>MTVQMEYEKDVKVAALDGKKIAVIGYGSQGHAHAQNLRDSGRDVIIGVRPGKSFDKAKEDGFDTYTVAEATKLADVIMILAPDEIQQELYEAEIAPNLEAGNAVGFAHGFNIHFEFIKVPADVDVFMCAPKGPGHLVRRTYEEGFGVPALYAVYQDATGNAKNIAMDWCKGVGAARVGLLETTYKEETEEDLFGSQAVLCGGLTALIEAGFEVLTEAGYAPELAYFEVLHEMKLIVDLIYEGGFKKMRQSISNTAEYGDYVSGPRVITEQVKEN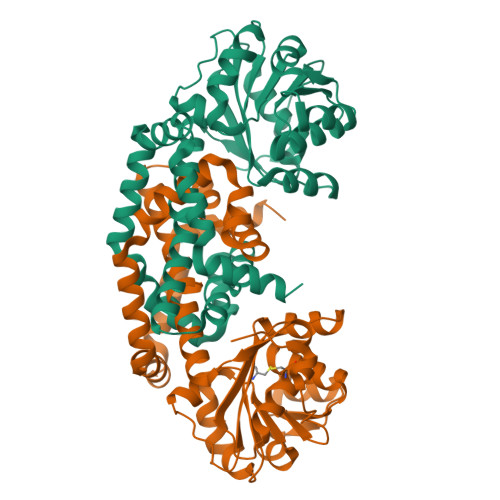MKAVLADIQNGKFANDFVNDYKAGRPKLTAYREQAANLEIEKVGAELRKAMPFVGKNDDDAFKIYN[2x]> PNSMKNIESLFDYSAGQFEFIDHLLTMGVGVHFAALIFFLVVSQFVAPKYRIATALSCIVMVSAGLILNSQAVMWTDAYAYVDGSYQLQDLTFSNGYRYVNWMATIPCLLLQLLIVLNLKGKELFSTATWLILAAWGMIITGYVGQLY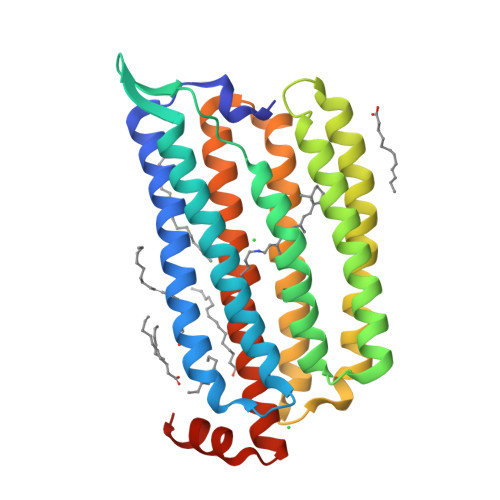EVDDIAQLMIWGAVSTAFFVVMNWIVGTKIFKNRATMLGGTDSTITKVFWLMMFAWTLYPIAYLVPAFMNNADGVVLRQLLFTIADISSKVIYGLMITYIAIQQSAAAGYVPAQQALGRIGMDSKAA>[2x]SHMSKYKHTVINNSVTLVLGDAIQIASLLPKCILVNAANRHLKHGGGIAGVINKASGGDVQEESDEYISNNGPLHVGDSVLLKGHGLADAILHVVG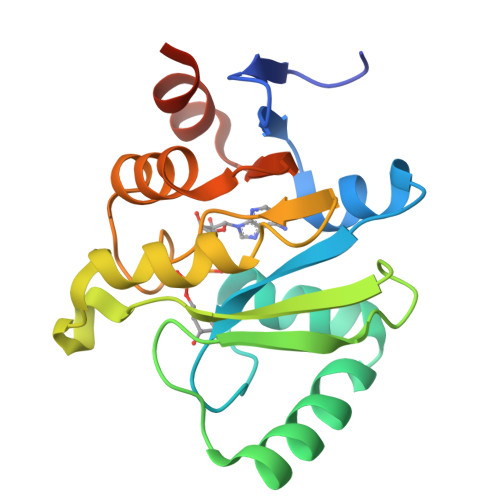PDARNNEDAALLKRCYKAFNKHTIVVTPLISAGIFSVDPKVSFEYLLANVTTTTYVVVNNEDIYNTLATPSKPDGLVY> KEAAPLQYLRPGMVLLKKFLKHDDQVDIIRRCQKLGIGSGGFYTPGYRDGGKLSLQM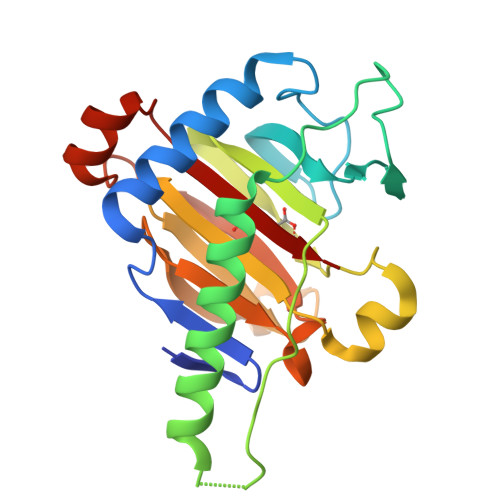MCLGKNWDPNSRSYGDTRPFDGAQPPSIPEVFSKIVKDAIQASNEFLRQKARPANDVEELPPLSPDICLVNFYTSSGKLGLHQDKDETKPSLHKGLPVVSFSLGDTAEFLYGDVNDVDKASKVDLESGDVLIFGGKSRLIFHGVSRIKPKTAPNWLTDEAKLRPGRLNLTFRQH> GSAAASPAWMPAYACQRPTPLTHHNTGLSEALEILAEAAGFEGSEGRLLTFCRAASVLKALPSPVTTLSQLQGLPHFGEHSSRVVQELLEHGVCEEVERVRRSERYQTMKLFTQIFGVGVKTADRWYREGLRTLDDLREQPQKLTQQQKAGLQHHQDLSTPVLRSDVDALQQVVEEAVGQALPGATVTLTGGFRRGKLQGHDVDFLITHPKEGQEAGLLPRVMCRLQDQGLILYHQHQHSCCESPTRLAQQSHMDAFERSFCIFRLPQPGSWKAVRVDLVVAPVSQFP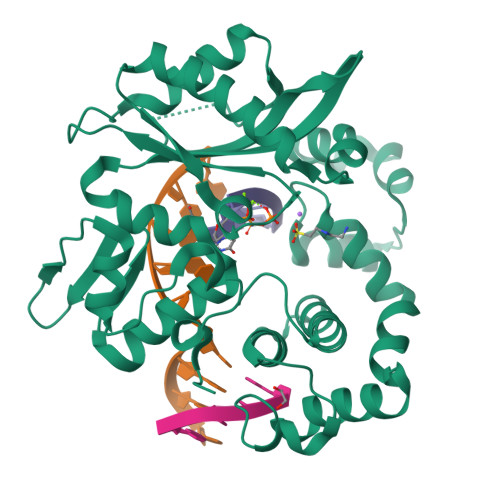FALLGATGSKLFQRELRRFSRKEKGLWLNSHGLFDPEQKTFFQAASEEDIFRHLGLEYLPPEQRNA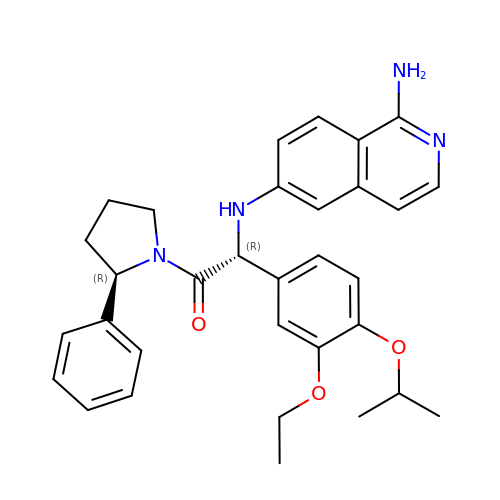2-[(1-aminoisoquinolin-6-yl)amino]-2-(3-ethoxy-4-propan-2-yloxyphenyl)-1-(2-phenylpyrrolidin-1-yl)ethanone | C32 H36 N4 O3 | ICHSQGVMXMADMI-POURPWNDSA-N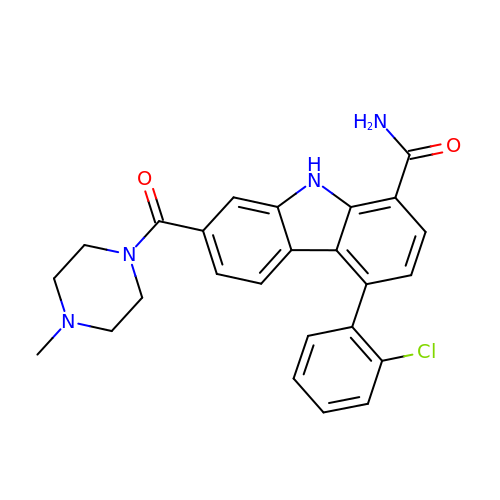4-(2-chlorophenyl)-7-[(4-methylpiperazin-1-yl)carbonyl]-9H-carbazole-1-carboxamide | C25 H23 Cl N4 O2 | YICBVOVZLQDBBM-UHFFFAOYSA-N> GAMGSMDIIQGLIQQPKIQSVDETIPTLCDRVENSTLISDRRSAVLGLKAFSRQYRESVIASGLKPLLNTLKRDYMDEDSVKAILETILILFIRGDGHDDLTRGWISQQSRLQNGKYPSPLVMKQEKEQVDQFSLWIADALTQSEDLIHLLVEFWEIDNFHIRLYTIQLLEAVMATRPLKARSALISLPTSISTMVSLLDDMHEPIRDEAILLLMAVVNDSPHVQKLVAFENIFERLFSIIEEEGGLRGSLVVNDCLSLINNILKYNTSNQTLFLETGNLPKLAHLLSEPISQDEVFFWNDQRIVNINTALDIVSLTVEPGNTVTTKHQNALLDSSVLMVVLRLAFFHNIPKKVRPVALLTAANMVRSNEHAQLEFSKIDVPYFDPSLPVNSTANGGPIKLIPVVSILINWMLYANSVHTFDTRVACSRLLKAYFMDNFDLQRDFLLKQVQLCNNSTNNVGDNAKENGGSNKSDKESDSDKDTDGKDGTEYEGSFKANLFEVLLNYDAELNLNPFKLFFTTDIFMFFFQQDHKYSEELREITRNVTTGNDLEDEEPLKAIQTISELLTTSLTAADIRIPISYLTFLIYWLFGDFKATNDFLSDKSVIKSLLSFSYQIQ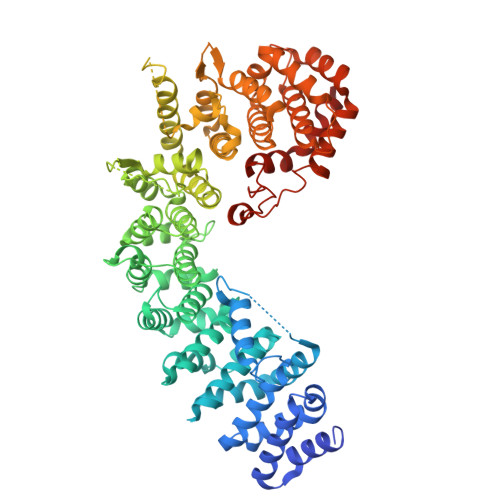DEDVTIKCLVTMLLGVAYEFSSKESPFPRKEYFEFITKTLGKDNYASRIKQFKKDSYFSKVDMNEDSILTPELDETGLPKVYFSTYFIQLFNENIYRIRTALSHDPDEEPINK> GPLGSMSTKTNIQKDWEQREFIEDMSINIQKIVEFLNKFELSTRNKLSDLNEKLTILDRQVDYLEATFKTVQE

The Scar/WAVE subunit is kept inactive by various interactions within the Scar/WAVE-complex, which consists of the five subunits Nap/Hem, Pir/Sra/CyFip, Abi, Scar/WAVE and Brk1/HSPC300, in a 1∶1∶1∶1∶1 stoichiometry. Brk1 is important for the stability of the Scar/WAVE subunit in different organisms, and was proposed to function as a precursor for Scar/WAVE-complex assembly in Hela S cells. Dictyostelium DdBrk1 encompasses 68 residues and shares 37% sequence identity and 52% similarity with human Brk1/HSPC300 (HsBrk1). Here we present the high resolution structure and a biochemical analysis of DdBrk1, which provides new insights on the question of how Brk1 may function as a precursor during the assembly of the mature Scar/WAVE-complex.

As DdBrk1 does not contain any methionines that could be used for selenomethionine substitution, and no molecular replacement model was available, we co-crystallized DdBrk1 in presence of heavy atom salts and collected a 1.5 Å resolution data set of platinum soaked crystals at Pt-peak wavelength. As DdBrk1 was crystallized in presence of 0.2 M Ca2+-ions, it is very likely that the anomalous signal of calcium at platinum peak-wavelength was sufficient for phasing of the relatively small protein due to the high resolution data and high multiplicity of the measurement. Thus, the refinement of the dataset of the native crystal was performed including two Ca2+-ions. The final model depicted in Figure 3A–C containing one DdBrk1-molecule in the asymmetric unit (residues 3–65), two molecules of MPD, two Ca2+-ions and 107 solvent molecules was refined to an R-value of 0.159 (Rfree = 0.182) and showed very good geometry. The DdBrk1-chain forms a single continuous α-helix and assembles into a triple-coiled-coil (left handed superhelix) with its symmetry molecules along a conserved hydrophobic patch. This triple-helix is stabilized via typical knobs-into-holes interactions with heptad-repeats of lysine residues with an interface area of 935Å2 between the single helices. Hydrogen bonds between Q55 of one chain and D57/E60 in the neighboring chain further stabilize the C-terminal triple-coil domain like a ring, as also observed in the structure of the actin-binding protein coronin 1. As the helix shows an approx. 20° bend at K33, residues 3–32 are opening up the triple-coil to form a funnel shaped N-terminal region. The entry into the triple-coil structure is highly hydrophobic and occupied by larger hydrophobic residues with additional stacking interactions (F30, F34). Residues 33–65 fold into a compact triple-coil structure whereas the missing residues of the N-terminus are probably flexible and thus can not be seen in the electron density.> MERNKLARQIIDTCLEMTRLGLNQGAAGNVSVRYQDGMLITPTGIPYEKLTESHIVFIDGNGKHEEGKLPSSEWRFHMAAYQSRPDANAVVHNHAVHCTAVSILNRSIPAIHYMIAAAGGNSIPCAPYATFGTRELSEHVALALKNRKATLLQHHGLIACEVNLEKALWLAHEVEVLAQLYLTTLA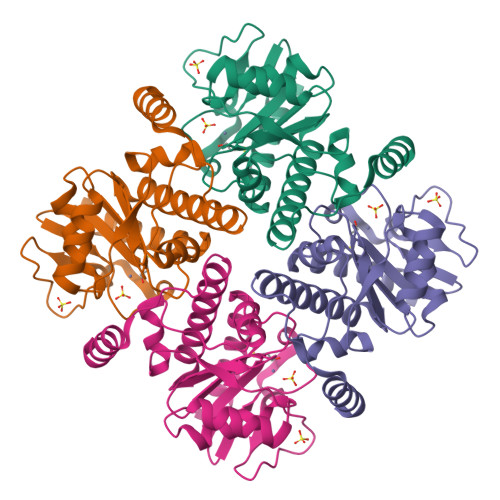ITDPVPVLSDEEIAVVLEKFKTYGLRIEE> GYSDRVEQITLGNSTITTQEAANSIVAYGEWPSFLSDVDASDVNKTTKPDTSACRFYTLDSKMWTQGSKGWCWKLPDALKDMGIFGQNMFFHSQGRTGYTIHVQCNATKFHSGCLLVVVIPEHQLASAEGGNVSVLYDKTHPGEKGIDLSEADSTGPMKDPLYMMDGTLIGNSLIFPHQFINLRTNNTATIVVPYINSVPMDSMTRHNNLSLMVIPIVDITATSGTTP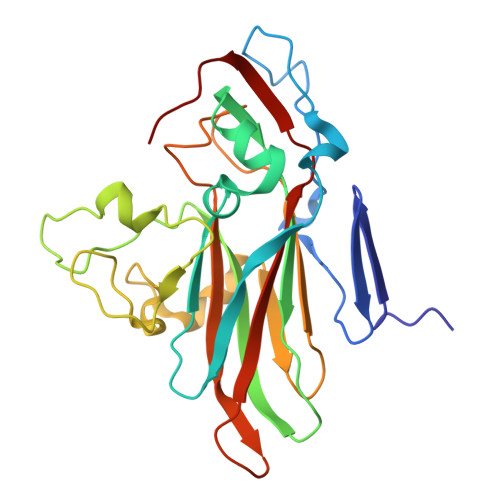SIPVTITIAPMFLELSGIRSKAVI> GSPLPAAGFKKQQRKFQYGNYCKYYGYRNPSCEDGRLRVLKPEWFRGRDVLDLGCNVGHLTLSIACKWGPSRMVGLDIDSRLIHSARQNIRHYLSEELRLPPQT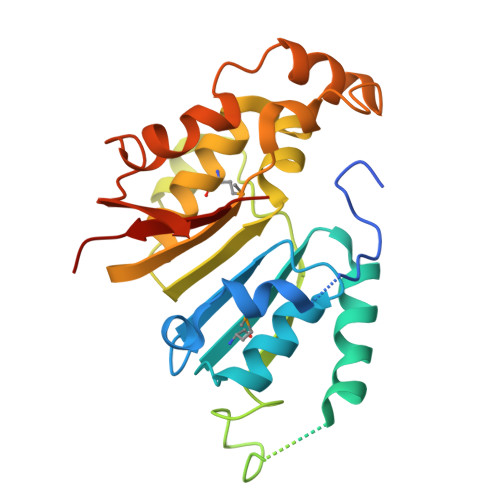LEGDPGAEGEEGTTTVRKRSCFPASLTASRGPIAAPQVPLDGADTSVFPNNVVFVTGNYVLDRDDLVEAQTPEYDVVLCLSLTKWVHLNWGDEGLKRMFRRIYRHLRPGGILVLEPQPWSSYGKRKTLTETIYKNYYRIQLKPEQFSSYLTSPDVGFSSYELVATPHNTSKGFQRPVYLFHKARSPSH> GGUUGACAAGAAACGAGUAACUCGUCCCUCUUCUGCAGACUGCUUACGGUUUCGUCCGUGUUGCAGUCGAUCAUCAGCAUACCUAGGUUU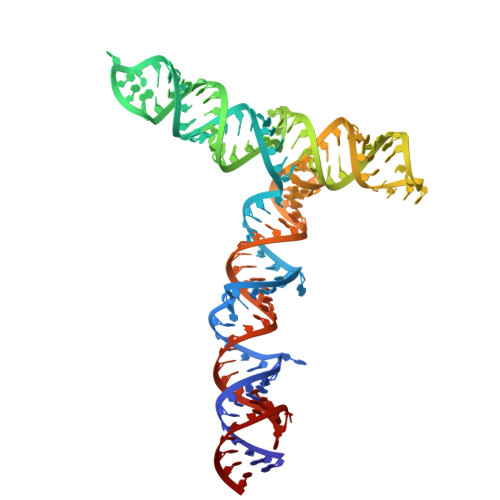CGUCCGGGUGUGACCGAAAGGUAAGAUGGAGAGCCUUGUUCUUGGUGUCAACC> 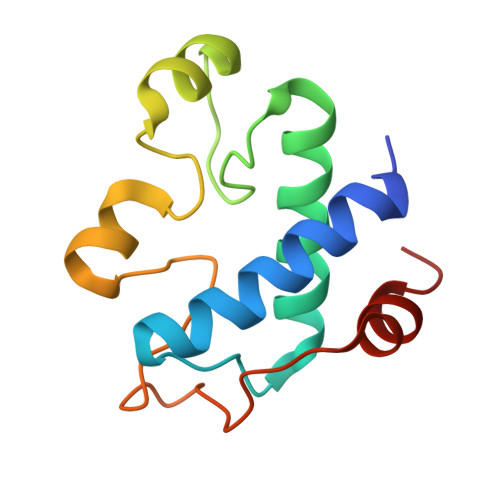AKTEPSEKSVEIMRKFSEQYARRSGTYFCVDKGVTSVVIKGLAEHKDSYGAPLCPCRHYDDKAAEVGQGFWNCPCVPMRERKECHCMLFLTPDNDFAGKDQTITSDEIKETTANM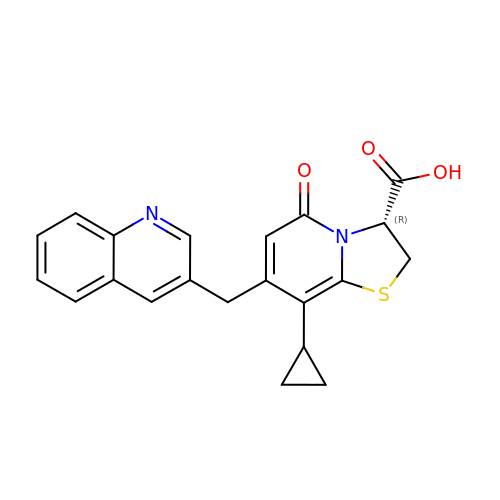(3~{R})-8-cyclopropyl-5-oxidanylidene-7-(quinolin-3-ylmethyl)-2,3-dihydro-[1,3]thiazolo[3,2-a]pyridine-3-carboxylic acid | C21 H18 N2 O3 S | UNLLRJXHYGIZSR-KRWDZBQOSA-N Leucine aminopeptidase (LAP) is found in all kingdoms of life and catalyzes the metal-dependent hydrolysis of the N-terminal amino acid residue of peptide or amino acyl substrates. We report here the X-ray structures of three kinetoplastid acidic LAPs (LAP-As from Trypanosoma brucei, Trypanosoma cruzi, and Leishmania major) which were solved in the metal-free and unliganded forms, as well as in a number of ligand complexes, providing insight into ligand binding, metal ion requirements, and oligomeric state. LAPs of the M17 family of aminopeptidases are bilobal proteins with a highly conserved C-terminal domain harboring the aminopeptidase activity. They form homohexamers of approximately 330 kDa with the active sites facing a central cavity separated from the bulk solvent but accessible through solvent channels.

The holo TbLAP-A (crystallized in the presence of leucine), TbLAP-A complexes, and LmLAP-A structures have two metals bound in the active site; the TcLAP-A structures, in contrast, clearly show only one metal ion in site 1 and no metal in site 2. In TbLAP-A, the carboxylate oxygen atoms of D294 and E373 and the main-chain and carboxylate oxygens of D371 coordinate the metal ion in site 1 and the carboxylate oxygens of D294, E373, and D312 and the ε-amino group of K289 coordinate that in site 2. Most LAP-A crystals were grown in the presence of manganese ions. As LAPs are reported to be zinc-dependent enzymes, crystals of EDTA-treated TbLAP-A were grown in the presence of ZnCl2. Nevertheless, X-ray fluorescence (XRF) scans of the resulting crystals indicated the presence of manganese ions, suggesting that EDTA may not to be able to efficiently chelate the Mn2+ ions at the concentrations used. A second data set was collected from the same crystal at a wavelength of 1.3052 Å, between the absorption edges of manganese and zinc, and an anomalous difference Fourier synthesis was calculated for the data sets at both wavelengths by using phases from the refined model. The map for the 1.3052-Å wavelength data showed peaks at around 10 σ for both metal sites, substantially larger than the 7 σ peaks for the original data recorded with a wavelength of 0.97949 Å, clearly indicating that neither site was occupied by zinc. The metals were therefore modeled as manganese ions.

>[12x]MPTLPKAEAKELSAFVQSCVEYKTNVCFTDVAAYESNQKGVLSSGLAVLVGTHKQLRDPAVQRLPFYNPAVAEAIERVKEGGTYGVLVEGLANAAGSKFVRVVVGEVPTKASRNNCPARPDVVTALVTAALDEVKEPNTTVDVFVLSNAVLPIAAAVARCGKHNFSAKDGAAAAAYNSGKVSRLQVVFPEPPAIPPKDLEAVATSTQLCQRLVDAPPNLLTTATFTEIAQGYAKALGFDVDVICGDDLCERGYGGIYSVGKAAFEAPRLVTLLYTPKGTPVKKVSLVGKGIVYDCGGLALKPADYMKLMKHDMGGAAAVFCGFLTAVRLQQPVQLSCTLCLAENAIGPKSYRNDDIIVMKSGKTVEVINTDAEGRIVLGDGVFHATNELSFTPDVVIDMATLTGAQGIATGRHHAGLYVNEEGAEAAMLRAGRESGETCFPVLYCPEYHEPEFKSNHADMTNLMERRDNAGVSCAGYFITTHLSPKFTGAHIHVDLAYPVFNSNGATGFGPALLTEYFRKL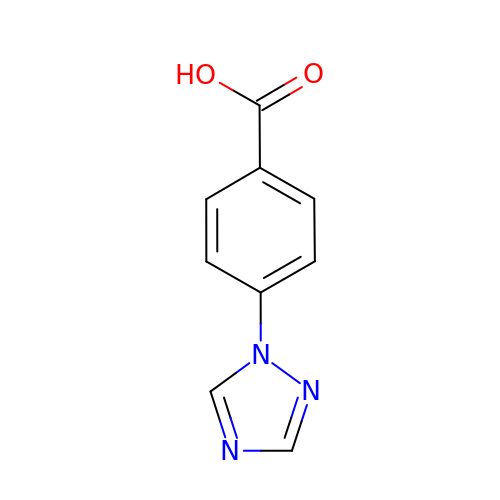4-(1H-1,2,4-triazol-1-yl)benzoic acid | C9 H7 N3 O2 | FOMQQGKCPYKKHQ-UHFFFAOYSA-N>[12x]MSEYIRVTEDENDEPIEIPSEDDGTVLLSTVTAQFPGACGLRYRNPVSQCMRGVRLVEGILHAPDAGWGNLVYVVNYPKDNKRKMDETDASSAVKVKRAVQKTSDLIVLGLPWKTTEQDLKEYFSTFGEVLMVQVKKDLKTGHSKGFGFVRFTEYETQVKVMSQRHMIDGRWCDCKLPNSKQSQDEPLRSRKVFVGRCTEDMTEDELREFFSQYGDVMDVFIPKPFRAFAFVTFADDQIAQSLCGEDLIIKGISVHISNAEPKHNSNRQLERSGRFGGNPGGFGNQGGFGNSRGGGAGLGNNQGSNMGGGMNFGAFSINPAMMAAAQAALQSSWGMMGMLASQQNQSGPSGNNQNQGNMQREPNQAFGSGNNSYSGSNSGAAIGWGSASNAGSGSGFNGGFGSSMDSKSSGWGM

The transactive response DNA-binding protein-43 (TDP-43) is a multi-facet protein involved in phase separation, RNA-binding, and alternative splicing. In the context of neurodegenerative diseases, abnormal aggregation of TDP-43 has been linked to amyotrophic lateral sclerosis and frontotemporal lobar degeneration through the aggregation of its C-terminal domain. Here, we report a cryo-electron microscopy (cryo-EM)-based structural characterization of TDP-43 fibrils obtained from the full-length protein. We found three different fibril structures in our sample that share the same basic fibril protein fold and differ in the number and relative arrangement of the fibril protofilaments.

Morphology-1 has a width of 11.5 ± 0.8 nm and well-resolved cross-overs at a distance of 46.9 ± 4.5 nm (n = 50). Subjecting the cryo-EM images of Morphology-1 to a reconstruction of the three-dimensional (3D) map resulted in the subdivision of the extracted fibril segments during 3D classification. The two distinct 3D classes were identified and refined. We hereafter refer to these two structures as Morphologies-1a and 1b. The 3D maps reached spatial resolutions of 3.76 Å (Morphology-1a) and 4.05 Å (Morphology-1b), based on the 0.143 Fourier Shell Correlation (FSC) criterion. Morphology-1a is C2-symmetrical and consists of two structurally equal, in-register protein stacks. In the case of both Morhphology-1a and 1b, extra densities were observed near the contact sites of two protofilaments. We find that the majority (~66%) of the fibrils visible in our micrographs are mixed and contain segments from both structural forms. The segments of the two structural forms are not randomly scattered throughout the mixed fibrils but occur clustered into distinct z-axial regions of variable length. These features imply that Morphologies-1a and 1b do not represent systematically distinct fibril morphologies but sub-morphologies that are able to coexist in mixed fibrils. Despite these differences, we find the interfaces between the adjacent protein stacks to be formed by the same two amino acid residues (Met311 and Phe313) in the three fibrils.>[2x]MEEPEEPADSGQSLVPVYIYSPEYVSMCDS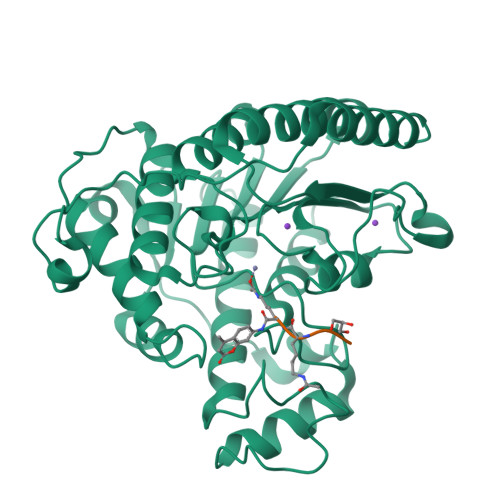LAKIPKRASMVHSLIEAYALHKQMRIVKPKVASMEEMATFHTDAYLQHLQKVSQEGDDDHPDSIEYGLGYDCPATEGIFDYAAAIGGATITAAQCLIDGMCKVAINWSGGWAHAKKDEASGFCYLNDAVLGILRLRRKFERILYVDLDLHHGDGVEDAFSFTSKVMTVSLHKFSPGFFPGTGDVSDVGLGKGRYYSVNVPIQDGIQDEKYYQICESVLKEVYQAFNPKAVVLQLGADTIAGDPMCSFNMTPVGIGKCLKYILQWQLATLILGGGGFNLANTARCWTYLTGVILGKTLSSEIPDHEFFTAYGPDYVLEITPSCRPDRNEPHRIQQILNYIKGNLKHVVIEGRGSHHHHHH> MDPQGDAAQKTDTSHHDQDHPTFNKITPNLAEFAFSLYRQLAHQSNSTNILFSPVSIAAAFAMLSLGAKGDTHDEILEGLNFNLTEIPEAQIHEGFQELLHTLNQPDSQLQLTTGNGLFLSEGLKLVDKFLEDVKKLYHSEAFTVNFGDTEEAKKQINDYVEKGTQGKIVDLVKELDRDTVFALVNYIFFKGKWERPFEVKDTEEEDFHVDQVTTVKVPMMKRLGMFNIQHSKKLSSWVLLMKYLGNATAIFFLPDEGKLQHLENELTHDIITKFLENEDRRSASLHLPKLSITGTYDLKSVLGQLGITKV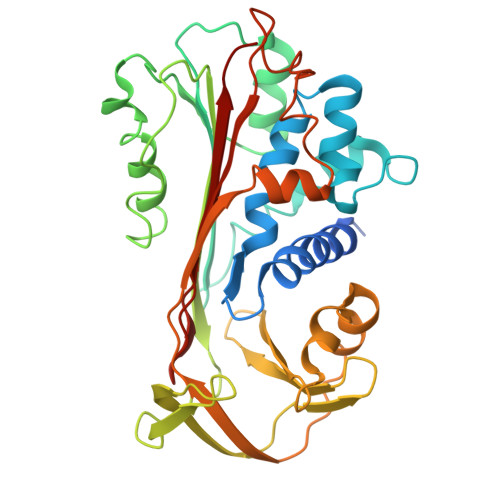FSNGADLSGVTEEAPLKLSKAVHKAVLTIDEKGTEAAGAMFLEAIPM>MSVLNTPNHYKMDNSGRRVVIDPVTRIEGHMRCEVNVDENNVIQNAVSTGTMWRGLEVILRGRDPRDAWAFVERICGVCTGCHALASVRAVEDALDIKIPHNATLIREIMAKTLQIHDHIVHFYHLHALDWVNPVNALKADPQATSELQKLVSPHHPMSSPGYFKDIQIRIQKFVDSGQLGIFKNGYWSNPAYKLSPEADLMAVTHYLEALDFQKEIVKIHAIFGGKNPHPNYMVGGVPCAINIDGDMAAGAPINMERLNFVKSLIEQGRTFNTNVYVPDVIAIAAFYRDWLYGGGLSATNVMDYGAYPKTPYDKSTDQLPGGAIINGDWGKIHPVDPRDPEQVQEFVTHSWYKYPDETKGLHPWDGITEPNYELGSKTKGSRTNIIEIDESAKYSWIKSPRWRGHAVEVGPLARYILAYAQGVEYVKTQVHTSLNRFNAVCRLLDPNHKDITDLKAFLGSTIGRTLARALESEYCGDMMLDDFNQLISNIKNGDSSTANTDKWDPSSWPEHAKGVGTVAAPRGALAHWIVIEKGKIKNYQCVVPTTWNGSPRDPKGNIGAFEASLMGTPMERPDEPVEVLRTLHSFDPCLACSTH[2x];>[2x]NKIAHAMETKPRTPVIWLHGLECTCCSESFIRSAHPLAKDVVLSMISLDYDDTLMAASGHAAEAILDEIKEKYKGNYILAVEGNPPLNQDGMSCIIGGRPFSEQLKRMADDAKAIISWGSCASWGCVQAAKPNPTQATPVHKFLGGGYDKPIIKVPGCP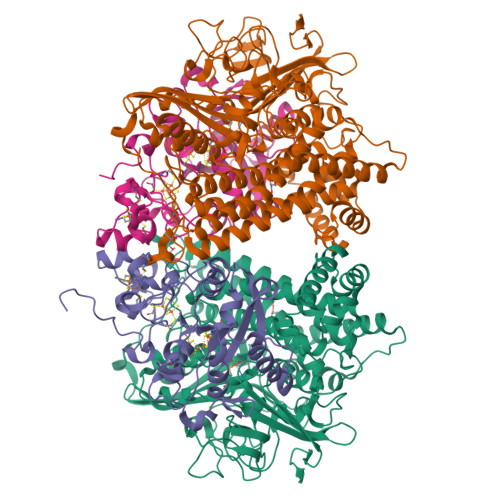PIAEVMTGVITYMLTFDRIPELDRQGRPKMFYSQRIHDKCYRRPHFDAGQFVEEWDDEGARKGYCLYKVGCKGPTTYNACSTVRWNGGTSFPIQSGHGCIGCSEDGFWDKGSFYSRDTEMNAFG> IVGGYECKAYSQPHQVSLNSGYHFCGGSLVNENWVVSAAHCYKSRVEVRLGEHNIKVTEGSEQFISSSRVIRHPNYSSYNIDNDIMLIKLSKPATL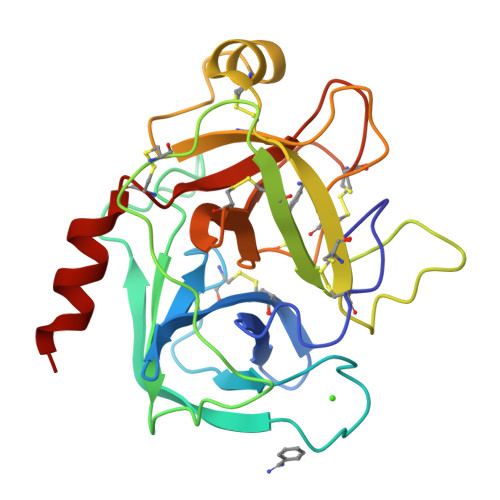NTYVQPVALPTSCAPAGTMCTVSGWGNTMSSTADSNKLQCLNIPILSYSDCNNSYPGMITNAMFCAGYLEGGKDSCQGDSGGPVVCNGELQGVVSWGYGCAEPGNPGVYAKVCIFNDWLTSTMASY>[44x]MALNSINTNSGA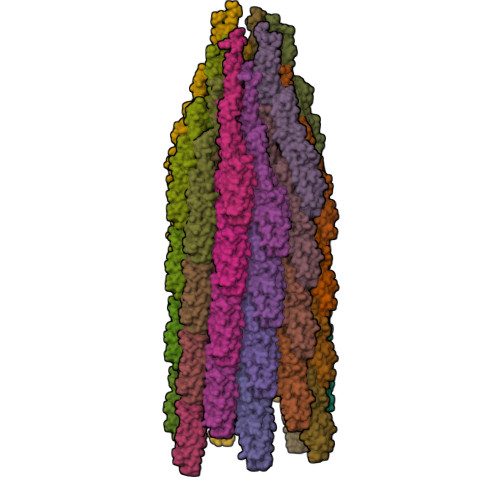LIALQNLNSTNAELTQVQQRINTGKKIGSAKDNGAIWATAKNQSATANSMNAVKDSLQRGQSTIDVALAAGDTITDLLGKMKEKALAASDTSLNTASFNALKSDFDSLRDQITKAASNAKFNGVSIANGSTAKLTFLANSDGSGFTVTAKTLTLTGLGLTASSTFTTAAAAKTMIGTIDTALQTATNKLASLGTSSTGLDTHLTFVGKLQDSLDAGVGNLVDADLAKESAKLQSLQTKQQLGVQALSIANSSSSAILSLFR>[2x]XGFVC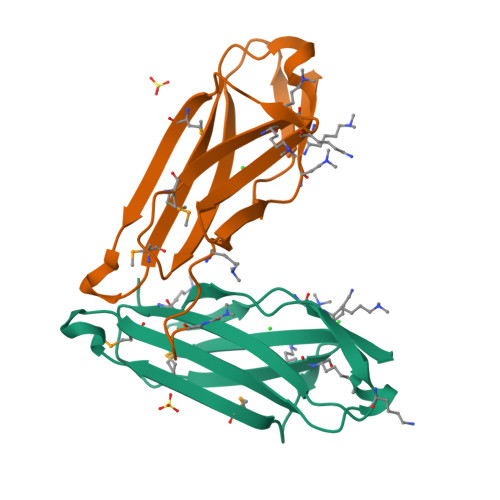DDFPKPQITVQPETQSAIKGSDVSFTCSAASSSDSPMTFAWKKDNEALQDAEMENYAHLRAQGGELMEYTTILRLRNVEFTSEGKYQCVISNHFGSSYSVKAKLTIN> MVTIMHIEELLDIEDHGERDRQLRRYLAPYSAEIGVDGAEKMALVVLLNLTLKRDRVESLCDEGLARQLL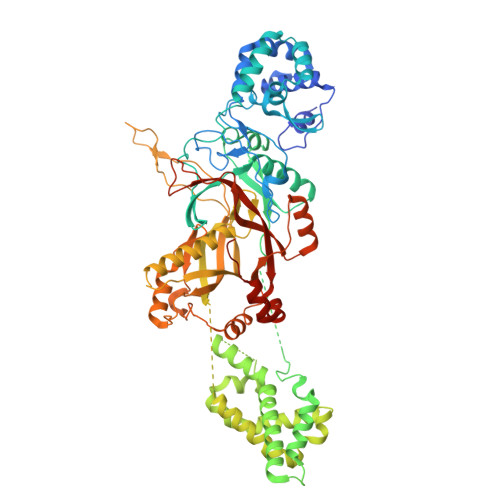SDEGHITNCLHTVRWLHTHNLKYPDARVSGERLIINAPPLIPGVISSAGLPMRMGWAHDSSDINLAKLFGTSFRYRDDSTNLALQLVARSKTWEQALIGLGLTQQQLDIWCQLLASNLENNTFPTVVSPFSKQVRFLYQGNYCVVTPVVSHALLAQLQNVVHEKKLQCTYIHHDHPASVGSLVGALGGKVAVLDYPPPVSPDKARSFSQARKHRLANGQSLFDRSVFNDHVFIDALKHVISRPGLTRKQQRQLRLSALRYLRRQLAIWLGPIIEWRDEIVSSGRGEPGNLPSGGLELELITQPKKMLPELMLQVAGRFHLELQNHSAGRRFAFHPALMAPIKSQILWLLRQLADDEEKDEPHPPTSCYYLHLSGLTVYDASALANPYLCGIPSLSALAGFCHDYERRLQSLIGQSVYFRGLAWYLGRYSLVTGKHLPEPSKSADPKSVSAIRRPGLLDGRYCDLGMDLIIEVHIPTGGSLPFTTCLDLLRVALPARFAGGCLHPPSLYEEYNWCTVYQDKSTLFTVLSRLPRYGCWIYPSDADLRSFEELSEALALDRRLRPVATGFVFLEEPVERAGSIEGQHVYAESAIGTALCINPVEMRLAGKKRFFGAGFWQLNDAKGAILMNGSANTG> MSTTTTEARSPLPLLLRRGRSSTALSASTAEARSPLSILQFRRRSSKDVRNITSVSSSLLPAFGTFIEDDNPSSKPFIVLHFDRRYRLWELFLVILVGYSAWASLFELAFEKAAEGALLTIDLVVDFFFAVDIILTFFVSYLDNTTYLNVTDHKLIAKRYLKSVAFVMDVASTLPIQFIYKTITGDVGRGQAFGFLNLLRLWRLRRVAELFKRLEKDAHFNYFVIRVIKLLCVTIFWIHLAGCILYWIAYHYPRPTDTWIGSQVEDFKERSVWLGYTYSMYWSIVTLTTVGYGDLHAVNSREKTFNMFYMLFNIGLTSYIIGIMTNLVVHGALRTFAMRSAINDILRYTSKNRLPDTMREQMLAHMQLKFKTAELRQEEVLQDLPKAIRSSINQHLFRSIIEEAYLFKGFPEGLLVQLVSQIQAEYFPPKMEIILQNEIPTDFYVIVSGGVDIIASKGVSEQVLAKLGPGSMAGEIGVVFNIPQPFTVRTRRLSQVIRIGHHKFKEMVQSDNDVDAKMIIANFMTYLKGLND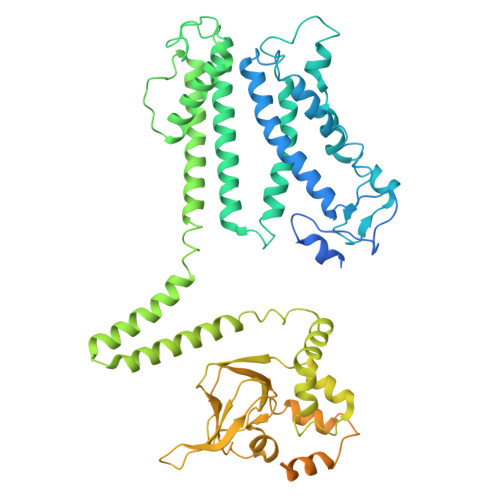ELKKEIPFLRDLLDDADAQVQETVQSEETPQSNDEEIVTVSRHENGQIEERRREGVPKRVIIHGQAPPNQDNKNNGDSNGRLIILPDSIQLLFDLAEKKLGKRGSTIAMADGAHVEQIDALRENDHLYIFLEGSDEVDAGSAAASGGSGSWSHPQFEK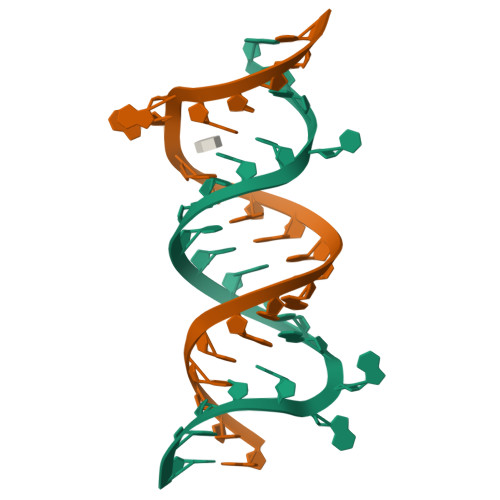>[2x]GCGUCACACCGGUGAAGUCGC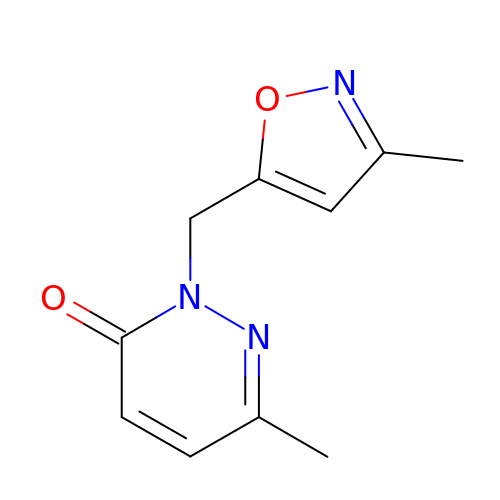6-methyl-2-[(3-methyl-1,2-oxazol-5-yl)methyl]pyridazin-3(2H)-one | C10 H11 N3 O2 | PLCLGFAKZPXQFY-UHFFFAOYSA-N> ASMYLKEIFVDNFRNLKKQKLEFCEGVNLIYGLNAQGKSNLLEAIRLLSMGRSFRGSKMSELVKFDEEYFYVRGLVRSADFYEKKIEFGYKVNGNKVIKVNGNKLKSTGEILGHFLTVIFSPEDIEIIKEGPSRRRKYLDACISVIDKNYFFDLLQYNKTLSNRNSLLKKIKEEGKGEDLLEIFDEKLAEYGARIIKVRNNYLEKLKNSMSKFLMEISNEKLEIIYLNSAGVKEVHEENLIREKLKNRLTKSLTLDLKYLSTQVGPHREDFKILINGYDSRVYSSQGQKRTAALCLKLSELEILEEETGEKPVLLLDDVMSELDDNRKKYILKKLEGFQSFITHTSKSDVEGDCCFKIYDGIVDKLA

RecF is a multifunctional protein involved in recombinant DNA repair, homologous genetic recombination, and DNA replication. Similar to RecR and RecO, RecF is a recombination mediator protein (RMP) in the RecFOR pathway for ssDNA gap repair. RecF contains the conserved Walker A motif, Walker B motif and signature motif of ABC-ATPase that exhibits ATP-dependent dimerization; additionally, the signature motif residues interact with the ATP bound to the opposite molecule. To gain insight into the mechanism of ABC-ATPase RecF, we solved the crystal structures of TTERecF, TTERecF-ATP, and TTERecF-ATPɤS.

The results of size-exclusion chromatography demonstrated that in solution, TTERecF (42 KDa) forms a monomer, whereas TTERecF-ATP (84 KDa) and TTERecF-ATPɤS (84 KDa) form a dimer. The structure of TTERecF consisted of two domains. Domain II contained six α-helices (αB, αC, αD, αE, αF, and αG) and two β-sheets (β7 and β8), in which the signature motif was the loop between β8 and αG. Domain II is similar to Lobe II subdomain of Rad50 and SMC protein; however, in the Rad50 and SMC proteins, helices corresponding to αD and αE extended into a long coiled-coil region, which was absent in TTERecF. Comparison of the structures of the ATP-free TTERecF and one monomer of the ATP-bound TTERecF dimer showed that the two monomers were similar. The root mean square deviation (r.m.s.d) was 1.015 Å under Cα trace superimposition. Notably, two structures differed in terms of their conservative Walker A motif and Walker B motif. In ATP-free TTERecF, the last turn (residues 35–38) of the helix αA in the Walker A motif occupied the ATP binding site, whereas in the binding of ATP with TTERecF, the last turn was flipped by 180° relative to the ATP-free TTERecF to create a space for ATP to further interact with TTERecF. Moreover, the helix αH of Walker B motif moved by 4 Å relative to the ATP-free TTERecF. The KD values of the TTERecF monomer interacting with the 21mer ssDNA and dsDNA were 576 nM and 1.63 µM, respectively, however, the TTERecF-ATP dimer binding 21mer ssDNA and dsDNA showed KD values of 16 nM and 6.2 nM, respectively.>[2x]VSKRAVITGLGIVSSIGNNQQEVLASLREGRSGITFSQELKDSGMRSHVWGNVKLDTTGLIDRKVVRFMSDASIYA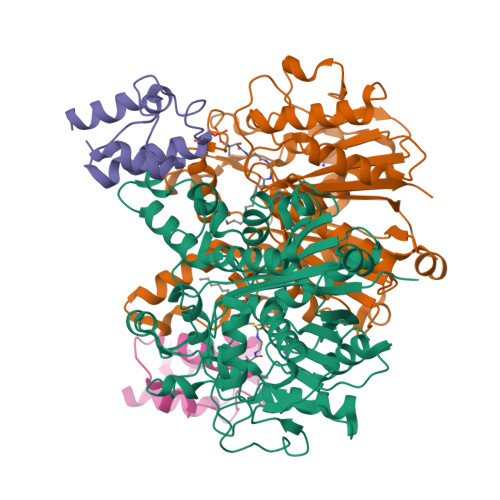FLSMEQAIADAGLSPEAYQNNPRVGLIAGSGGGSPRFQVFGADAMRGPRGLKAVGPYVVTKAMASGVSACLATPFKIHGVNYSISSACATSAHCIGNAVEQIQLGKQDIVFAGGGEELCWEMACEFDAMGALSTKYNDTPEKASRTYDAHRDGFVIAGGGGMVVVEELEHALARGAHIYAEIVGYGATSDGADMVAPSGEGAVRCMKMAMHGVDTPIDYLNSHGTSTPVGDVKELAAIREVFGDKSPAISATKAMTGHSLGAAGVQEAIYSLLMLEHGFIAPSINIEELDEQAAGLNIVTETTDRELTTVMSNSFGFGGTNATLVMRKLK;>[2x]STIEERVKKIIGEQLGVKQEEVTNNASFVEDLGADSLDTVELVMALEEEFDTEIPDEEAEKITTVQAAIDYINGHQA> MKNKQHVAIFPFPFGSHLPPLLNLVLKLAHIAPNTSFSFIGTHSSNAFLFTKRHIPNNIRVFTISDGIPEGHVPANNPIEKLDLFLSTGPDNLRKGI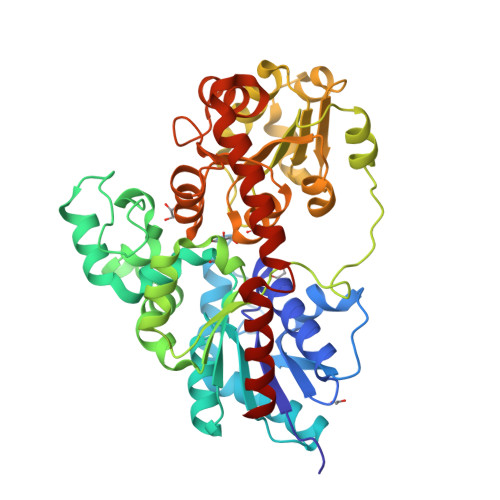ELAVAETKQSVTCIIADAFVTSSLLVAQTLNVPWIAFWPNVSCSLSLYFNIDLIRDKCSKDAKNATLDFLPGLSKLRVEDVPQDMLDVGEKETLFSRTLNSLGVVLPQAKAVVVNFFAELDPPLFVKYMRSKLQSLLYVVPLPCPQLLLPEIDSNGCLSWLDSKSSRSVAYVCFGTVVSPPPQEVVAVAEALEESGFPFVWALKESLLSILPKGFVERTSTRGKVVSWVPQSHVLSHGSVGVFVTHCGANSVMESVSNGVPMICRPFFGDQGIAARVIQDIWEVGVIVEGKVFTKNGFVKSLNLILVQEDGKKIRDNALKVKQIVQDAVGPHGQAAEDFNTLVEVISSS>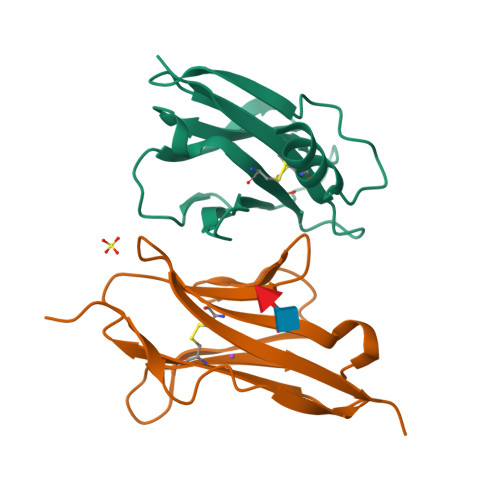 ADPASEEVMACLRQERSRVENPSQTIVNVVAENPAYLHCSVPPDAEHEIAWTRVSDGALLTAGNRTFTRDPRWQVSKKSANIWVLNLRRAEQQDSGCYLCEINDKHNTVYAVYLKVLEPHHHHHH;> GSGAPPTIQQPSMSSAVALLGQDVDFTCIVNDLGSHMVAFVKADSPPRLLSFDEKVFRRRNKYELKPRIGDLHNEWVLTIKNVQESDRGNYSCQINTEPITLSTGELDVKVPHHHHHH> MNTSVPTSVPTNQSVWGNVST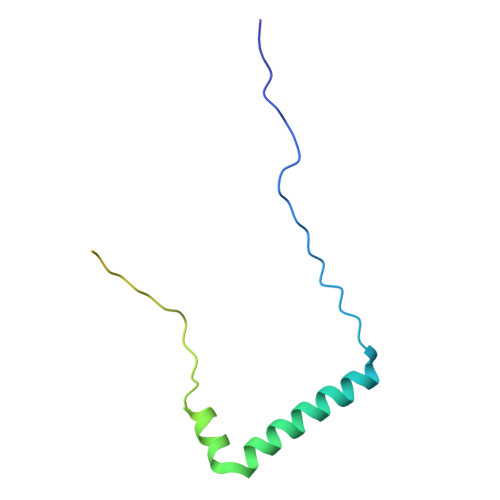GLDALISGWARVEQIKAAKASTGQGRVEQAMTPELDNGAAVVVEAPKKAAQPSETLVFGVPQKTLLLGFGGLLVLGLVMRGNK Vitamin D receptor (VDR) is a ligand-dependent transcriptional factor belonging to the nuclear receptor superfamily, and mediates most of the biological functions of vitamin D3, including calcium and phosphate homeostasis, bone metabolism, and immune regulation. The endogenous agonist of VDR is 1α,25-dihydroxyvitamin D3 [1α,25(OH)2D3, 1], an active metabolite of vitamin D3, which induces increased expression of target genes. Lithocholic acid (LCA, 2) is a secondary bile acid formed from chenodeoxycholate, and was identified as a second endogenous agonist of VDR. However, the lithocholic acid derivative 3 (Dcha-20) is a more potent agonist than 1α,25(OH)2D3, (1), and its carboxyl group has similar interactions to the 1,3-dihydroxyl groups of 1 with amino acid residues in the VDR ligand-binding pocket.

We next attempted X-ray crystallographic analysis of the complex of rat VDR LBD (residues 116–423, Δ165–211) with several of the lithocholic acid amide derivatives. According to the method reported in our previous study, a synthetic peptide containing the target sequence of the coactivator MED1 (mediator of RNA polymerase II transcription subunit 1, also known as ARC205 or DRIP205) was included in the crystallization solution of VDR LBD and the test compound. However, the analysis was successful only for the complex of compound 7b. The electron density map clearly shows the VDR LBD, the coactivator peptide, the ligand and a relatively low number of water molecules. Figure 5a shows the overall structure of the VDR LBD complex with 7b; it is similar to those previously reported for VDR LBD complexes with other lithocholic acid derivatives. The hydroxyl group in the 3-substituent of 7b forms direct hydrogen bonds with two histidine residues, His301 (O···N distance: 2.79 Å) and His393 (O···N distance: 2.68 Å). The direct interactions of the hydroxy group in the 3-substituent with two histidines may contribute to the potent activity of 7b and 3. The carboxyl group of compound 3 (Dcha-20) formed hydrogen bonds with the phenolic hydroxyl group of Tyr143 (O··O distance: 2.81 Å) in helix 1 and the hydroxymethyl group of Ser274 (O··O distance: 3.13 Å) in helices 4/5, whereas the amide group of 7b did not form a hydrogen bond with any amino acid residue. Instead, the terminal carboxyl group of 7b formed hydrogen bonds with Arg270 (O···N distance: 2.82 Å) and the backbone amide bond of Tyr143 (O···N distance: 2.91 Å). Among the synthesized amide derivatives, compounds 4a, 6 with an N-cyano group and 7b with an N-2-carboxyethyl group showed the most potent activity.

> GSHMGSPNSPLKDSLRPKLSEEQQHIIAILLDAHHKTYDPTYADFRDFRPPVRMDGSTGSVTLDLSPLSMLPHLADLVSYSIQKVIGFAKMIPGFRDLTSDDQIVLLKSSAIEVIMLRSNQSFTMDDMSWDCGSQDYKYDVTDVSKAGHTLELIEPLIKFQVGLKKLNLHEEEHVLLMAICIVSPDRPGVQDAKLVEAIQDRLSNTLQTYIRCRHPPPGSHQLYAKMIQKLADLRSLNEEHSKQYRSLSFQPENSMKLTPLVLEVFGNEIS;> KNHPMLMNLLKDN4-{4-(4-fluorophenyl)-1-[1-(1,2-oxazol-3-ylmethyl)piperidin-4-yl]-1H-imidazol-5-yl}pyrimidin-2-amine | C22 H22 F N7 O | 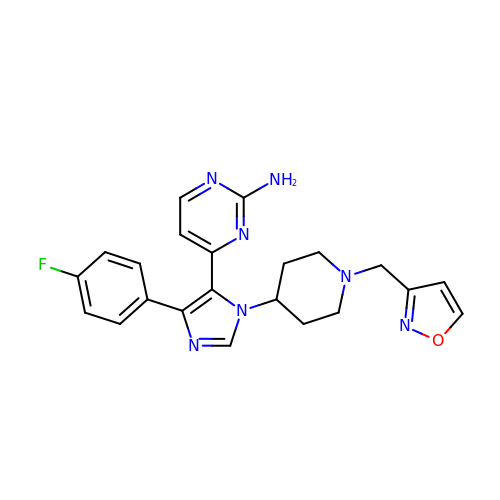XPWHRQHBPRSUAW-UHFFFAOYSA-N> GSHMSLSNKLTLDKLDVKGKRVVMRVDFNVPMKNNQITNNQRIKAAVPSIKFCLDNGAKSVVLMSHLGRPDGVPMPDKYSLEPVAVE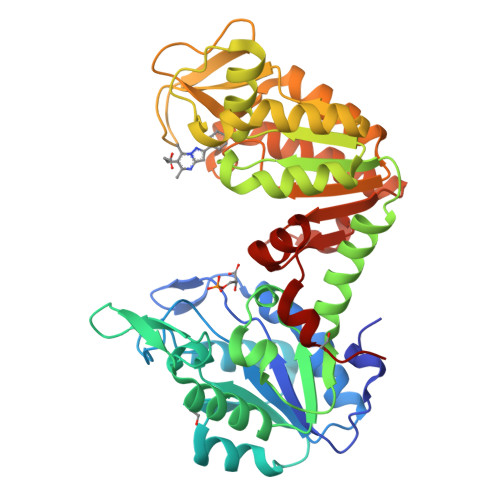LKSLLGKDVLFLKDCVGPEVEKACANPAAGSVILLENLRFHVEEEGKGKDASGNKVKAEPAKIEAFRASLSKLGDVYVNDAFGTAHRAHSSMVGVNLPQKAGGFLMKKELNYFAKALESPERPFLAILGGAKVADKIQLINNMLDKVNEMIIGGGMAFTFLKVLNNMEIGTSLFDEEGAKIVKDLMSKAEKNGVKITLPVDFVTADKFDENAKTGQATVASGIPAGWMGLDCGPESSKKYAEAVTRAKQIVWNGPVGVFEWEAFARGTKALMDEVVKATSRGCITIIGGGDTATCCAKWNTEDKVSHVSTGGGASLELLEGKVLPGVDALSNI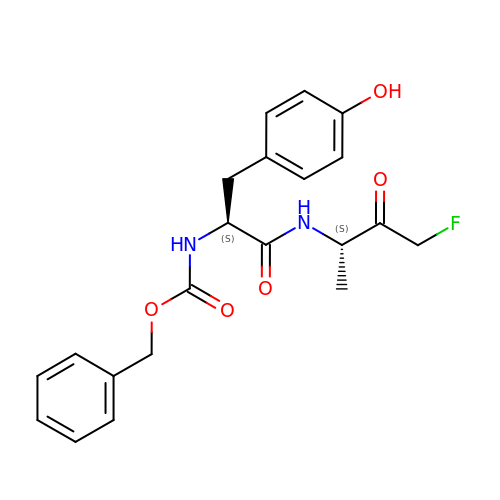BENZOYL-TYROSINE-ALANINE-FLUORO-METHYL KETONE | C21 H23 F N2 O5 | RYABQRLJLIHDIP-KSSFIOAISA-N> MKILGISGGMRNGSNDGMCIEALMGAKEMGAEVEFIQLQNLHIEHCTGCTACVQSVLGGRGGKCVLKDDFDWLLDKMLDADGIVFSTPIFEKGATGLFHTITDRFGPRMDRGNNIIGTKIAEETGGTAPDPRILKDKVISFMSVGGSDWVTRTQCDA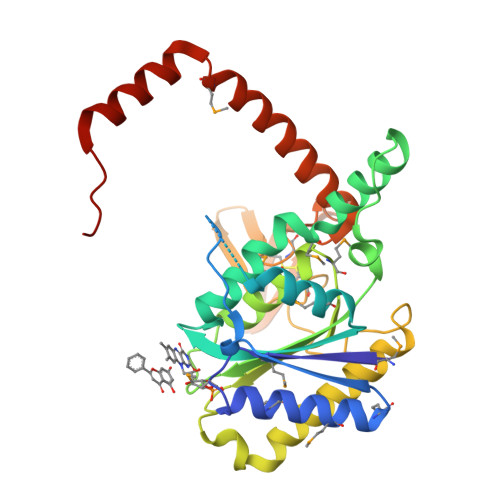GMLALTPMWKVIDNEVFPWALSILVEDERVARAHQIGRNIAEAAKDIEHAQYQGDAGVCPHCHSRNFHLQDGKAICCLCGLEGEIHNEGGKYSFTFPAEQLEHAHDTLSGKFIHGNDIKENTGKKIANMQTEKYKARQAAYRAFITATVPEKG>[2x]GHMENKVINFKKIIDSRGSLVAIEENKNIPFSIKRVYYIFDTKGEEPRGFHAHKKLEQVLVCLNGSCRVILDDGNIIQEITLDSP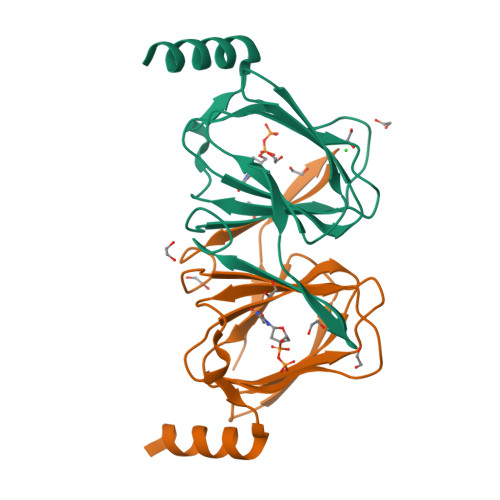AVGLYVGPAVWHEMHDFSSDCVMMVLASDYYDETDYIRQYDNFKKYIAKINLEKEG> MARLVLHEVRYVLMAMLYISRGMAKQIQNSTIDLYVYWFLTFIPIASLCVPQFTYLVVDTKSLIDFISVLVPITEILLTNGKMIICNVKRGKIINLINQVQVAWDECAKSEHLEIQTLITATAKKTKIFVIIYTTSFLLICVEYSSMPLFKLIYHSAVYGKQSNYTIALPYLSRFAYSTESTTSFAWTYFFILLGVYLLALTLSGFDSLFATLVMHVKMMFKVLKFEIEQLGLDLSAGKSHVELQAKLKQIILKHKTNLSLIEQLEDGFSFFLMAQFLTSSILVCVVLYELTMVFGWNEDTFKTVTYLPGAILQLFLFCWYAQQITEEARLVSDHIYNIPWYLADPKLQKDILTFMVKAQKPTGVTASKFYMVTLQTFQ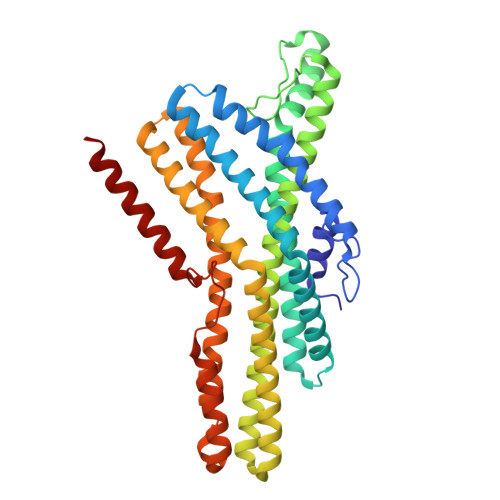RISSTSYSYFTLLQTINQQ(2Z)-N-(3-chloro-2'-methoxybiphenyl-4-yl)-2-cyano-3-hydroxybut-2-enamide | C18 H15 Cl N2 O3 | 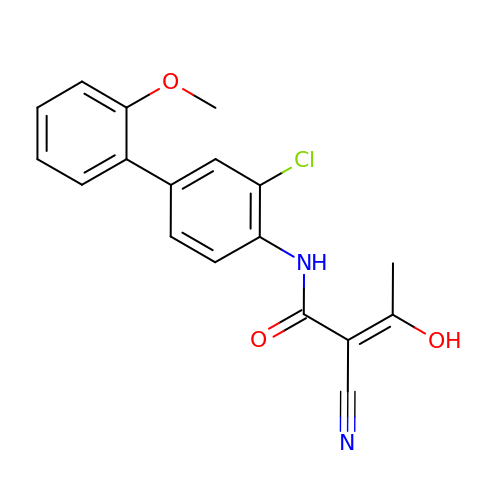YUDQXOMZBLEWBH-KAMYIIQDSA-N7-methoxy-8-(3-methylbut-2-enyl)chromen-2-one | C15 H16 O3 | 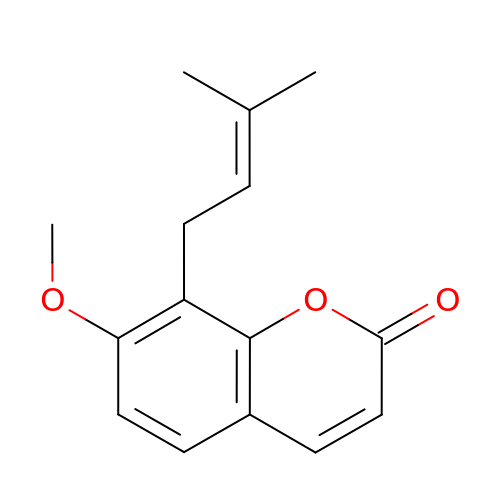MBRLOUHOWLUMFF-UHFFFAOYSA-N>MLTQHVSEARTRGAIHTARLIHTSDLDQETRDGARRMVIEAFRDPSGDSDFTDDFTDDDWDHALGGMHALISHHGALIAHGAVVQRRLMYRGPDGRGHALRCGYVEAVAVREDRRGDGLGTAVLDALEQVIRGAYQIGALSASDIARPMYIARGWLSWEGPTSVLTPTEGIVRTPEDDRSLFVLPVDLPDGLELDTAREITCDWRSGDPW[2x]

Three different classes of enzymes are well established: ATP-dependent phosphotransferases (O-phosphorylation, APH), ATP-dependent nucleotidyltransferases (O-nucleotidylation, ANT), and acetyl coenzyme A (CoA)-dependent N-acetyl-transferases (N-acetylation, AAC). Here, we present the crystal structures of an AAC(2′) from M. smegmatis [AAC(2′)-Id] in its apo-form and AAC(2′)-Id complexed with CoA and different aminoglycosides (gentamicin, sisomicin, neomycin, and paromomycin). Collectively, the kinetic results indicate that AAC(2′)-Id has a very broad substrate-binding specificity, similar to AAC(2′)-Ic9. AAC(2′)-Id was not active on streptomycin because the antibiotic does not contain 2′ amino groups in its chemical structure, indicating that AAC(2′)-Id exhibits strict regioselectivity.

Sisomicin is structurally similar to gentamicin but has a unique unsaturated diamino sugar at the ring I position. In the sisomicin-CoA-AAC(2′)-Id complex structure, the overall interaction mode of sisomicin is identical to that of gentamicin, except for an additional hydrogen bond formed between the main chain carbonyl group of Asp54 and the second amino group on ring I of sisomicin. However, three ring-containing aminoglycosides (4,6-disubstituted aminoglycosides: gentamicin and sisomicin) bind toward the β8–β9 loop region and make several interactions with this loop, whereas four ring-containing aminoglycosides (4,5-disubstituted aminoglycosides: neomycin and paromomycin) bind toward the α1–α2 loop region and make several interactions with it. In our activity assay data, AAC(2′)-Id showed a stronger binding affinity and more catalytic efficiency to three ring-containing aminoglycosides (gentamicin and sisomicin) than four ring-containing aminoglycosides (neomycin and paromomycin). It is thought that three ring-containing-aminoglycosides form additional hydrophobic interactions with the β8–β9 loop as well as the β5–α4 loop. Comparison analysis between gentamicin and sisomicin complex structures indicated that interaction between gentamicin and AAC(2′)-Id is stronger than that between AAC(2′)-Id and sisomicin. Unlike sisomicin, gentamicin contains methyl groups connected to the 6′ and amine group in ring I. The methyl group of 6′ forms a hydrophobic interaction with F42 and F55, and the other methyl group connected to the amine group interacts with the D59 backbone and probably influence the shift of the 45–53 loop region toward gentamicin and cover the active site. Consistent with this observation, the turnover rate of AAC(2′)-Id for gentamicin is slower than that for sisomicin. Our biochemical analysis revealed that AAC(2′)-Id can bind to various aminoglycoside antibiotic substrates, with a strong preference for sisomicin.(2S)-1-bromopropan-2-ol | C3 H7 Br O | 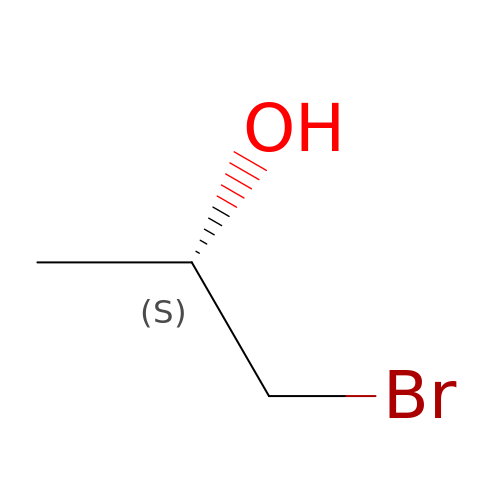WEGOLYBUWCMMMY-VKHMYHEASA-N> 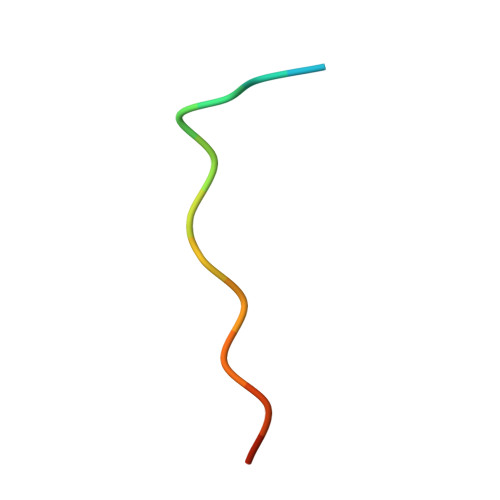SNLNPNAKEFVPGVK> MIETPYLLFLGDAPDMLAAKVAIGIRDWRPDHAVGQISLPGCGANLGLTEMTLEEAKAAGAKTLVIGVANRGGKISQEWKKVLVQALEEGFDLASGLHNLLRDEPDLAAVAEATGRTLHDVRVPSVQYPIADGVKRRGKRCLAVGTDCSVGKMYTALAMDAEMQARGIKSTFRATGQTGILITGDGVPLDAVIADFMAGSIEYLTPDNDDDHWDLIEGQGSLFHVSYSGVTM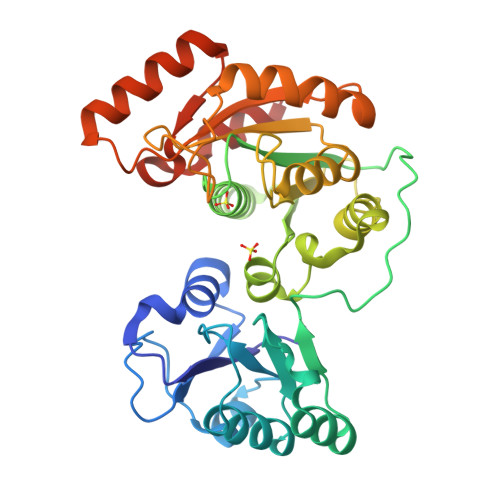ALVHGGQPDALILCHEPTRTHMRGLPDYDVPSLEELRDVALPLAQRANKDCKIVGISVNTQHLGEEEAVAYLKEVEGRMGLPAVDPYRHGAGRLVDALAAVLEHHHHHH> ESKKRQWALEDFEIGRPLGKGKFGNVYLAREKQSKFILALKVLFKAQLEKAGVEHQLRREVEIQSHLRHPNILRLYGY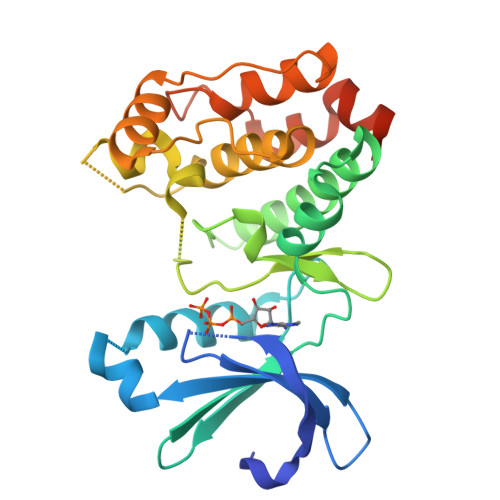FHDATRVYLILEYAPLGTVYRELQKLSKFDEQRTATYITELANALSYCHSKRVIHRDIKPENLLLGSAGELKIANFGWSVHAPSSRRTTLCGTLDYLPPEMIEGRMHDEKVDLWSLGVLCYEFLVGKPPFEANTYQETYKRISRVEFTFPDFVTEGARDLISRLLKHNPSQRPMLREVLEHPWITANSSKPSNCQNKESASKQS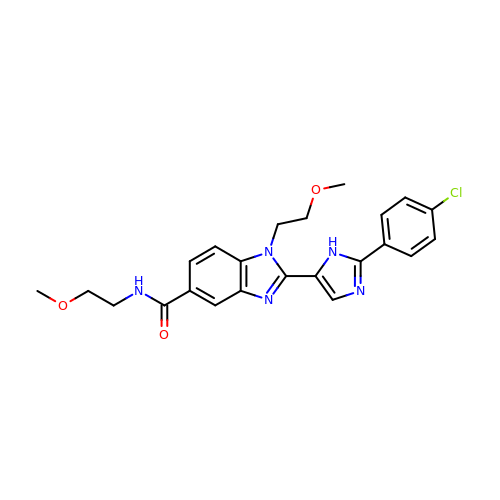2-(2-(4-CHLOROPHENYL)-1H-IMIDAZOL-5-YL)-N,1-BIS(2-METHOXYETHYL)-1H-BENZO[D]IMIDAZOLE-5-CARBOXAMIDE | C23 H24 Cl N5 O3 | GALXSGLZQVWBNV-UHFFFAOYSA-N> MRRLLFLSLAGLWLFSPAAAAQLPGLISQPLAGGGQSWSLSVQTLVFITSLTFLPAILLMMTSFTRIIIVFGLLRNALGTPSAPPNQVLLGLALFLTFFIMSPVIDKIYVDAYQPFSEQKISMQEALDKG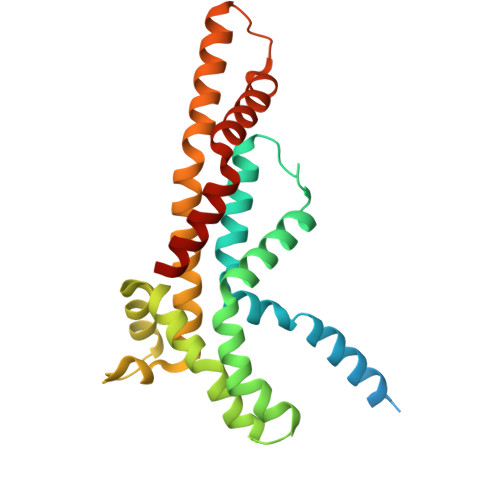AQPLRAFMLRQTREADLALFARLANSGPLQGPEAVPMRILLPAYVTSELKTAFQIGFTIFIPFLIIDLVIASVLMALGMMMVPPATIALPFKLMLFVLVDGWQLLMGSLAQSFYS> MTMV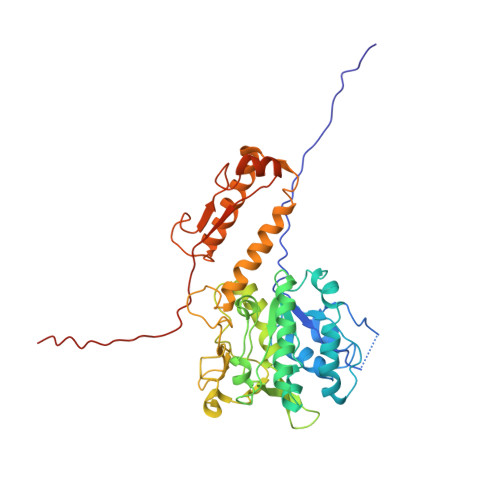LPGVSYNETLLTQASNDDPVTMPLFIGYTPPDTAIPVTVMQPVSVGSLTQANSLFGQRGTLAYSLRHFFENGGLQCYVLPLGPGKGEPAARLQELIAALQTPQMLETLLADDKTGLVLVPELSELNEVSSTSLSAEGVDAAEVDADALWYQGWQVLLTLCRQAPQRFALLELPEDPASAVTLTQQSFSADQCQRGAAWWPRLETSYQDESSAPVVLSPLPAVAAAIQRSAHDNGVWKAPANIALAKTRRPTQSILTSQALLDNQGVSCNLIRSFVGKGVRLWGCRTLLNEENTAWRYIQIRLLVSSVEHYLSKLARAYLFEPNTAPTWMKLKGQVWTWLRQQWLAGAFFGTVEDEAFSLSIGLDETMTEDDIRHGKMILQVRLALLAPAEFIAISLTLDLRDGTASAQTGGQS PUF proteins, named for PUM (Pumilio) and FBF (fem-3 binding factor), are an exemplary system for understanding the divergence of RNA recognition within eukaryotic RNA-binding protein families. Eight PUM repeats are arranged in a crescent shape with the RNA bound on the concave face of the protein. Each repeat contributes a trio of amino acid residues, termed a tripartite recognition motif (TRM), that directly contact the opposing RNA base. FBF recognizes a 9-nt motif, 5´-UGURNNAUA-3´, whereas PUF-8 binds an 8-nt sequence, 5´-UGUANAUA-3´.

The variant bears an SS/Y TRM at repeat R5, and this imparted the ability to bind to the 8-nt PBE RNA. We found that the FBF-2 variant with an SS/Y TRM preferentially bound to the PBE versus the FBE. To understand how variation of the FBF-2 R5 TRM converts binding preference to an 8-nt PBE RNA, we determined a crystal structure of the R5 SS/Y variant in complex with a PBE RNA and found that the Y364 residue in the R5 TRM stacks between bases A4 and A5, which positions FBF-2’s PUM repeat R5 opposite a single RNA base, A4. In a manner similar to PUM1, Y364 of the the SS/Y variant occupies the space of the middle base of the triple stack, which allows interactions of repeats R5 and R4 with bases 4 and 5, respectively. The two serine side chains (S363 and S367) contact the A4 base. S363 forms a van der Waals interaction at the C2 position, and S367 interacts via a water molecule at the N1 position. FBF-2 R5 SS/Y retained the same overall curvature in complex with an 8-nt as wildtype FBF-2 in complex with a 9-nt RNA. We conclude that the change in identity of the TRM residues is sufficient for the transformation of binding site length specificity. Additionally, the crystal structure of the SS/Y variant bound to the PRE showed poor density for the 8th nucleotide. FBF-2 R5 SS/Y bound equally well to either an A or G at position 4, similar to WT FBF-2, and the R5 AS/Y variant accommodated A4, G4 or U4.

> GSNNVLPTWSLDSNGEMRSRLSLSEVLDSGDLMKFAVDKTGCQFLEKAVKGSLTSYQKFQLFEQVIGRKDDFLKLSTNIFGNYLVQSVIGISLATNDDGYTKRQEKLKNFISSQMTDMCLDKFACRVIQSSLQNMDLSLACKLVQALPRDARLIAICVDQNANHVIQKVVAVIPLKNWEFIVDFVATPEHLRQICSDKYGSYVVSTIIEKLTADSMNVDLTSAAQNLRERALQRLMTSVTNRCQELATNEYANYIIQHIVSNDDLAVYRECIIEKCLMRNLLSLSQEKFASHVVEKAFLHAPLELLAEMMDEIFDGYIPHPDTGKDALDIMMFHQFGNYVVQCMLTICCDAVSGRRQTKEGGYDHAISFQDWLKKLHSRVTKERHRLSRFSSGKKMIETLANLRSTHPIYELQ> ACTKNAIAQTGFNKDKYFNGDVWYVTDYLDLEPDDAPKRYCAALAAGTASGKLKEALYHYDPKTQDTFYDVSELQVESLGKYTANFKKVDKNGNVKVAVTAGNYYTFTVMYADDSSALIHTCLHKGNKAAGDLYAVLNRNKDAAAGDKVKSAVSA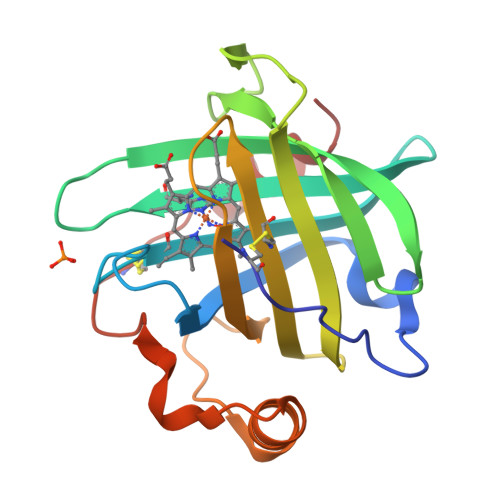ATLEFSKFISTKENNCAYDNDSLKSLLTK>MQNRLRSALALVTGAGSGIGRAVSVRLAGEGATVAACDLDRAAAQETVRLLGGPGSKEGPP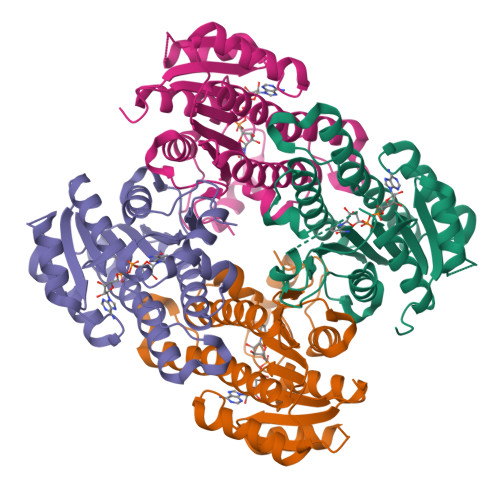RGNHAAFQADVSEARAARCLLEQVQACFSRPPSVVVSCAGITQDEFLLHMSEDDWDKVIAVNLKGTFLVTQAAAQALVSNGCRGSIINISSIVGKVGNVGQTNYAASKAGVIGLTQTAARELGRHGIRCNSVLPGFIATPMTQKVPQKVVDKITEMIPMGHLGDPEDVADVVAFLASEDSGYITGTSVEVTGGLFMAENLYFQ[4x]>HMLTMKDVIREGDPILRNVAEEVSLPASEEDTTTLKEMI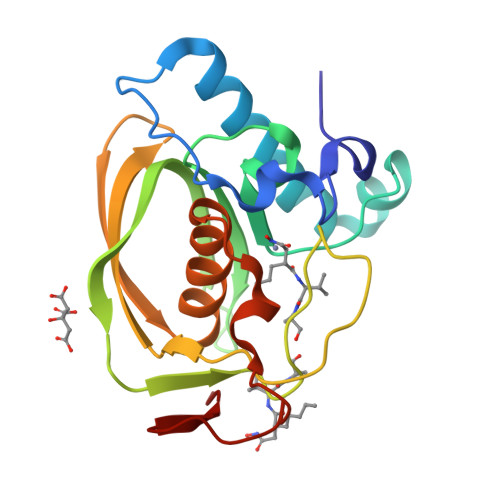EFVINSQDPEMAEKYSLRPGIGLAAPQIGVSKKMIAVHVTDADGTLYSHALFNPKIISHSVERTYLQGGEGCLSVDREVPGYVPRYTRITVKATSINGEEVKLRLKGLPAIVFQHEIDHLNGVMFYDHINKENPFAAPDDSKPLER[2x]> MALSRGLPRELAEAVAGGRVLVVGAGGIGCELLKNLVLTGFSHIDLIDLDTIDVSNLNRQFLFQKKHVGRSKAQVAKESVLQFYPKANIVAYHDSIMNPDYNVEFFRQFILVMNALDNRAARNHVNRMCLAADVPLIESGTAGYLGQVTTIK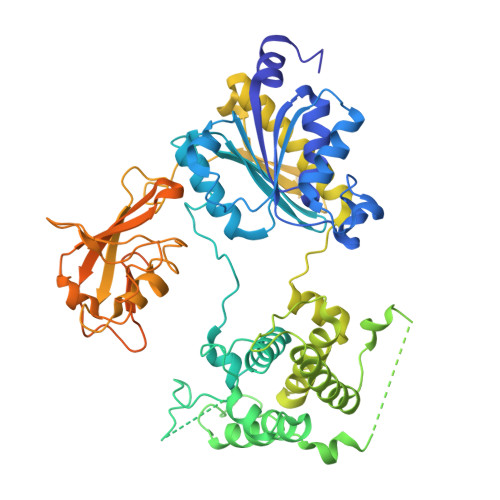KGVTECYECHPKPTQRTFPGATIRNTPSEPIHCIVWAKYLFNQLFGEEDADQEVSPDRADPEAAWEPTEAEARARASNEDGDIKRISTKEWAKSTGYDPVKLFTKLFKDDIRYLLTMDKLWRKRKPPVPLDWAEVQSQGEETNASDQQNEPQLGLKDQQVLDVKSYARLFSKSIETLRVHLAEKGDGAELIWDKDDPSAMDFVTSAANLRMHIFSMNMKSRFDIKSMAGNIIPAIATTNAVIAGLIVLEGLKILSGKIDQCRTIFLNKQPNPRKKLLVPCALDPPNPNCYVCASKPEVTVRLNVHKVTVLTLQDKIVKEKFAMVAPDVQIEDGKGTILISSEEGETEANNHKKLSEFGIRNGSRLQADDFLQDYTLLINILHSEDLGKDVEFEVVGDAPEKVGPKQAEDAAKSITNGSDDGAQPSTSTAQEQDDVLIVDSDEEDSSNNADVSEEERSRKRKLDEKENLSAKRSRIEQKEELDDVIALD> SLSNKLTLDKLNVKGKRVVMRVDFNVPMKNNQITNNQRIKAAVPSIKFCLDDGAKSVVLMSHLGRPDGSPMPDKYSLQPVAVELKSLLGKDVLFLKDCVGPEVEKACADPAAGSVILLENLRFHV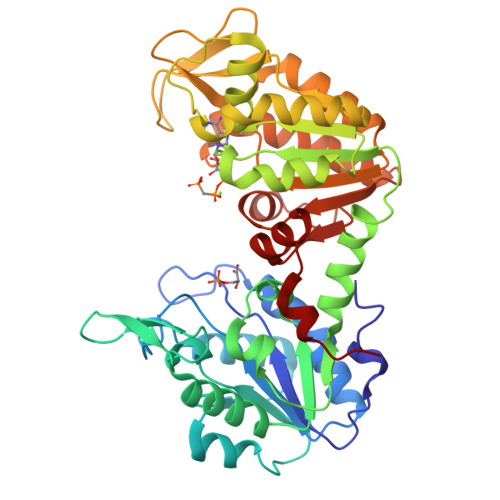EEEGKGKDASGNKVKAEPAKIKTFRASLSKLGDVYVNDAFGTAHRAHSSMVGVNLPKKAGGFLMKKELNYFAKALESPERPFLAILGGAKVADKIQLINNMLDKVNEMIIGGGMAFTFLKVLNNMEIGTSLFDEEGAKIVKNLMSKAEKNGVKITLPVDFVTADKFDEHAKTGQATVASGIPAGWMGLDCGPESSKKYSEAVARAKQIVWNGPVGVFEWEAFAQGTKALMDEVVKATSRGCITIIGGGDTATCCAKWNTEDKVSHVSTGGGASLELLEGKVLPGVDALSNV>[3x]MFNNEPLEQIDKELHDILADEEKRQRETINLIASENLTNGAVRECLGNRVSNKYSEGYPKKRYYGGNDFIDKIEELCQKRALEAFNVSDEEWGVNVQPLSGSAANVQALYALVGVKGKIMGMHLCSGGHLTHGFFDEKKKVSIT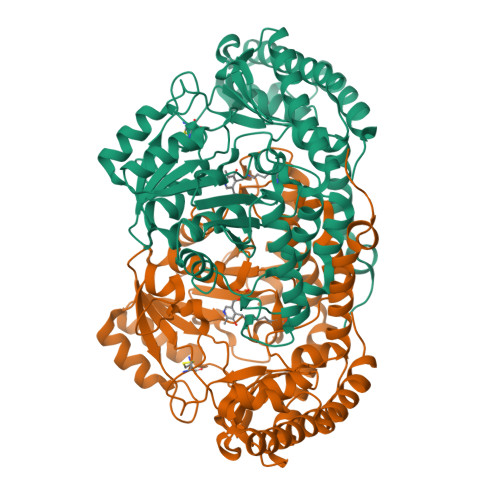SDMFESKLYKCNSQGYVDLDAVREMALSFKPKVIICGYTSYPRDIDYQQFRQICDEVNAYLFADISHISSFVACNILNNPFLHADVVTTTTHKILRGPRSALIFFNKKRNPGIEQKINSAVFPSFQGGPHNNKIAAVACQLKEVHSPAFKEYTQQVLLNSKALAKALISKQIDLVTNGTDNHLIVVDLRKFSITGSKLQETCNAINVSLNKNTIPSDVDCVSPSGVRIGTPAMTTRGAKEKDMEFIADVLARAIKITVDLQEQYGKKLVDFKKGLPGNAQLQQLKQEVVTWAGALPFP> GAGCAGACCTGA;> CGGCACTCA;> TCACCG;> TCTGAGTGGGT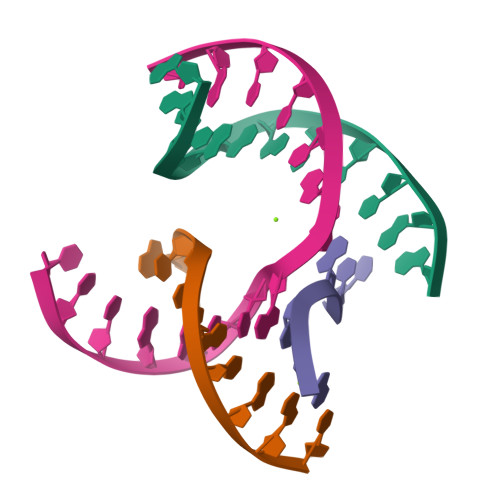CTGC>MTAPALSATAPAERCAHPGADLGAAVHAVGQTLAAGGLVPPDEAGTTARHLVRLAVRYGNSPFTPLEEARHDLGVDRDAFRRLLALFGQVPELRTAVETGPAGAYWKNTLLPLEQRGVFDAALARKPVFPYSVGLYPGPTCMFRCHFCVRVTGARYDPSALDAGNAMFRSVIDEIPAGNPSAMYFSGGLEPLTNPGLGSLAAHATDHGLRPTVYTNSFALTERTLERQPGLWGLHAIRTSLYGLNDEEYEQTTGKKAAFRRVRENLRRFQQLRAERESPINLGFAYIVLPGRASRLLDLVDFIADLNDAGQGRTIDFVNIREDYSGRDDGKLPQEERAELQEALNAFEERVRERTPGLHIDYGYALNSLRTGADAELLRIKPATMRPTAHPQVAVQVDLLGDVYLYREAGFPDLDGATRYIAGRVTPDTSLTEVVRDFVERGGEVAAVDGDEYFMDGFDQVVTARLNQLERDAADGWEEARGFLRLEHHHHHH[4x]

DesII is a radical S‐adenosyl‐l‐methione (SAM) enzyme that catalyzes the radical‐mediated deamination of TDP‐4‐amino‐4,6‐dideoxy‐d‐glucose (1) to TDP‐3‐keto‐4,6‐dideoxy‐d‐glucose (2) during the biosynthesis of TDP‐desosamine (3). Like other radical SAM enzymes, the catalytic cycle of DesII is characterized by initial single electron transfer from a reduced, active site [Fe4S4]+ cluster to SAM. Each monomeric unit comprises three domains: an N‐terminal domain of six α‐helices, a central radical SAM (RS) domain, and a C‐terminal domain consisting of a β‐hairpin and two α‐helices. The RS domain (residues S132–L369) coordinates the single [Fe4S4] cluster via residues C141, C145, and C148, which make up the CX3CX2C motif.

The present work reports the 2.33 Å crystal structure of DesII as a binary complex with SAM bound in the active site. The crystal structure of DesII from Streptomyces venezuelae was determined by single anomalous diffraction using a selenomethionine derivative. A single molecule of SAM was found coordinated to the [Fe4S4] cluster in chains a and c with methionine bound in the active sites of chains b and d. The C‐terminal His6‐tags of chains b and d were found to occupy the active site pockets of chains a and c, respectively. Four other previously identified SAM binding motifs including the GGE, ribose, GXIXGXXE, and β 6 motif are also conserved in DesII. The GGE motif (G187–E190) interacts with the Met moiety of SAM via H‐bonding interactions. In contrast, the R238, S240, and Y242 residues at the end of the β 4 strand H‐bond with the SAM ribose moiety to form the “ribose motif” originally described in BioB. The GXIXGXXE motif provides hydrophobic contacts to the adenine ring of SAM, which is further stabilized by backbone interactions with a polar residue in α 5 and hydrophobic interactions with Y324 as found in other radical SAM enzymes. Residue D323 in the loop behind the β 6 strand provides two backbone interactions with N1 and N6 of the adenine base, which is another feature of the β 6 motif. Molecular dynamics (MD) simulations and QM/MM computations were performed to evaluate the energetics of DesII‐catalyzed deamination of 1 based on the structure of the binary DesII·SAM complex.> MQRQALYRGLENREEVVGKIRSLHTDALKKLAVKCEDLFMAGQKDQLRFGVDSWSDFRLTSDKPCCEAGDAVYYTASYAKDPLNNYAVKICKSKAKESQQYYH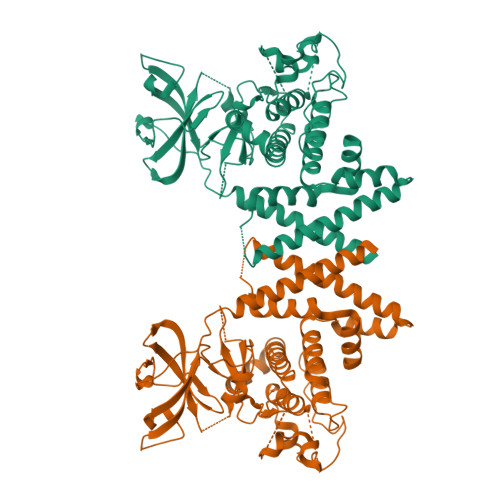SLAVRQSLAVHFNIQQDCGHFLAEVPNRLLPWEDPSKKQRSHVVVITREVPCLTVADFVRDSLAQHGKSPDLYERQVCLLLLQLCSGLEHLKPYHVTHCDLRLENLLLVHYQPGGTAQGFGPAEPTPTSSYPTRLIVSNFSQAKQKSHLVDPEILRDQSRLAPEIITATQYKKCDEFQTGILIYEMLHLPNPFDENPELKEREYTRADLPRIPFRSPYSRGLQQLASCLLNPNPSERILISDAKGILQCLLWGPREDLFQTFTACPSLVQRNTLLQNWLDIKRTLLMIKFAEKSLDREGGISLEDWLCAQYLAFATTDSLSCIVKILLEHHHHHH>MQKEPRKVREFRRREQEILDTALKLFLEQGEDSVTVEMIADAVGIGKGTIYKHFKSKAEIYLRLMLDYERDLAALFHSEDVARDKEALSRAYFEFRMRDPQRYRLFDRLEEKVVKTSQVPEMVEELHKIRASNFERLTQLIKERIADGKLENVPPYFHYCAAWALVHGAVALYHSPFWREVLEDQEGFFHFLMDIGVRMGNKRKREGD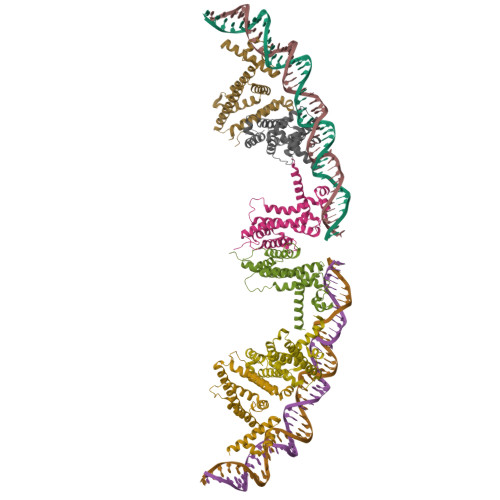APSA[6x]>[6x]MFSKLAHLQRFAVLSRGVHSSVASATSVATKKTVQGPPTSDDIFEREYKYGAHNYHPLPVALERGKGIY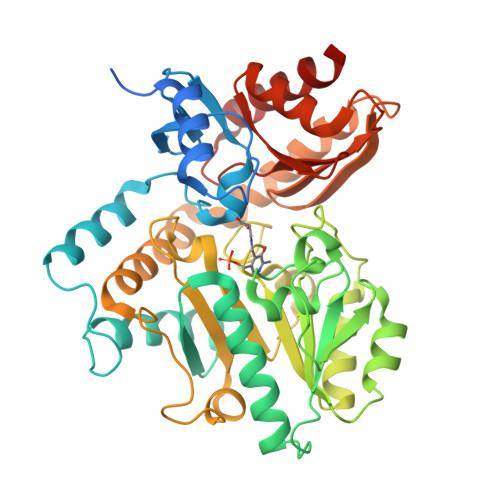LWDVEGRKYFDFLSSYSAVNQGHCHPKIVNALKSQVDKLTLTSRAFYNNVLGEYEEYITKLFNYHKVLPMNTGVEAGETACKLARKWGYTVKGIQKYKAKIVFAAGNFWGRTLSAISSSTDPTSYDGFGPFMPGFDIIPYNDLPALERALQDPNVAAFMVEPIQGEAGVVVPDPGYLMGVRELCTRHQVLFIADEIQTGLARTGRWLAVDYENVRPDIVLLGKALSGGLYPVSAVLCDDDIMLTIKPGEHGSTYGGNPLGCRVAIAALEVLEEENLAENADKLGIILRNELMKLPSDVVTAVRGKGLLNAIVIKETKDWDAWKVCLRLRDNGLLAKPTHGDIIRFAPPLVIKEDELRESIEIINKTILSF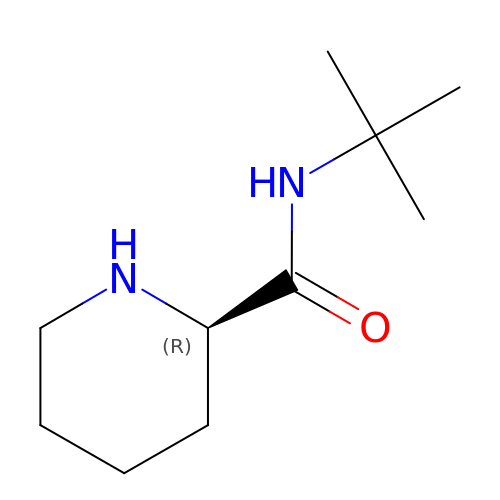(2R)-N-tert-butylpiperidine-2-carboxamide | C10 H20 N2 O | BZRGONFHSWNSQA-MRVPVSSYSA-N>MVLGKPQTDPTLEWFLSHCHIHKYPSKSTLIHQGEKAETLYYIVKGSVAVLIKDEEGKEMILSYLNQGDFIGELGLFEEGQERSAWVRAKTACEVAEISYKKFRQLIQVNPDILMRLSAQMARRLQVTSEKVGNLAFLDVTGRIAQTLLNLAK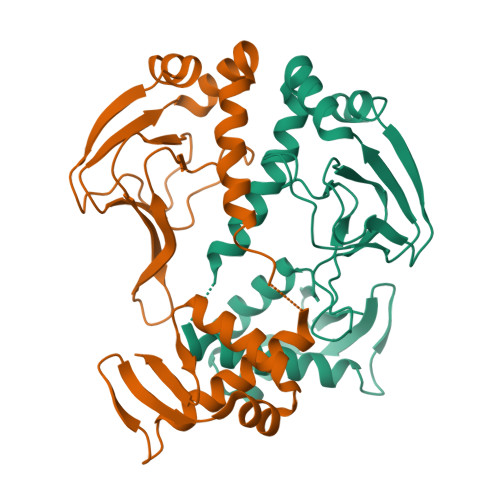QPDAMTHPDGMQIKITRQEIGQIVGCSRETVGRILKMLEDQNLISAHGKTIVVYGTR[6x]>MKHDYTNPPWNAKVPVQRAMQWMPISQKAGAAWGVDPQLITAIIAIQSGGNPNAVSKSNAIGLMQLKASTSGRDVYRRMGWSGEPTTSELKNPERNISMGAAYLNILETGPLAGIEDPKVLQYALVVSYANGAGALLRTFSSDRKKAI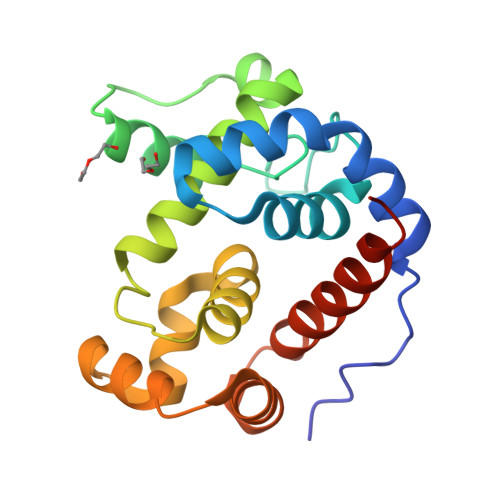SKINDLDADEFLEHVARNHPAPQAPRYIYKLEQALDAMLEHHHHHH[2x]>MLIAFEGIDGSGKTTQAKKLYEYLKQKGYFVSLYREPGGTKVGEVLREILLTEELDERTELLLFEASRSKLIEEKIIPDLKRDKVVILDRFVLSTIAYQGYGKGLDVEFIKNLNEFATRGVKPDITLLLDIPVDIALRRLKEKNEFENKEFLEKVRKG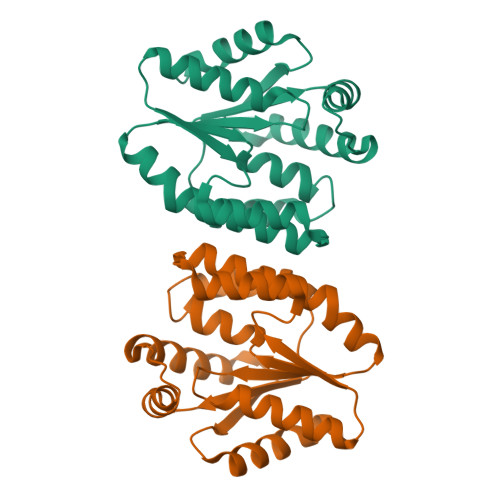FLELAKEEENVVVIDASGEEEEVFKEILRALSGVLRV[2x]> MNPIHDRTSDYHKYLKVKQGDSDLFKLTVSDKRYIWYNPDPKERDSYECGEIVSETSDSFTFKTVDGQDRQVKKDDANQRNPIKFDGVEDMSELSYLNEPAVFHNLRVRYNQDLIYTYSGLFLVAVNPFKRIPIYTQEMVDIFKGRRRNEVAPHIFAISDVAYRSMLDDRQNQSLLITGESGAGKTENTKKVIQYLASVAGRNQANGSGVLEQQILQANPILEAFGNAKTTRNNNSSRFGKFIEIQFNNAGFISGASIQSYLLEKSRVVFQSETERNYHIFYQLLAGATAEEKKALHLAGPESFNYLNQSGCVDIKGVSDSEEFKITRQAMDIVGFSQEEQMSIFKIIAGILHLGNIKFEKGAGEGAVLKDKTALNAASTVFGVNPSVLEKALMEPRILAGRDLVAQHLNVEKSSSSRDALVKALYGRLFLWLVKKINNVLCQERKAYFIGVLDISGFEIFKVNSFEQLCINYTNEKLQQFFNHHMFKVEQEEYLKEKINWTFIDFGLDSQATIDLIDGRQPPGILALLDEQSVFPNATDNTLITKLHSHFSKKNAKYEEPRFSKTEFGVTHYAGQVMYEIQDWLEKNKDPLQQDLELCFKDSSDNVVTKLFNDPNIASRAKKGANFITVAAQYKEQLASLMATLETTNPHFVRCIIPNNKQLPAKLEDKVVLDQLRCNGVLEGIRITRKGFPNRIIYADFVKRYYLLAPNVPRDAEDSQKATDAVLKHLNIDPEQYRFGITKIFFRAGQLARIEE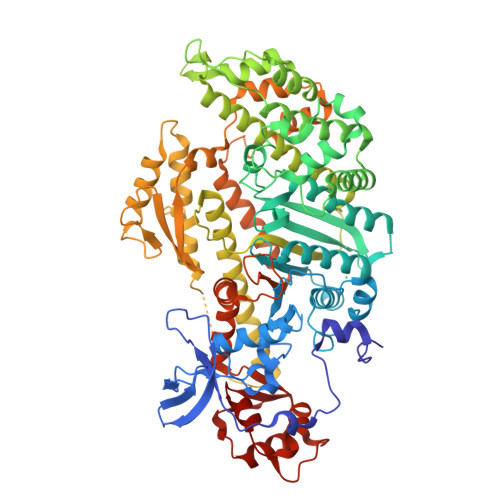AREPN> MAHHHHHHMPYQHIKVPEGGDKITVNKDFSLNVSDQPIIPYIEGDGTGFDITPVMIKVVDAAVEKAYGGKKKIHWMEIYAGEKATKVYGPDVWLPEETLQVLKEYVVSIKGPLTTPVGGGIRSLNVALRQELDLYVCLRPIQYFKGVPSPVREPEKTNMVIFRENSEDIYA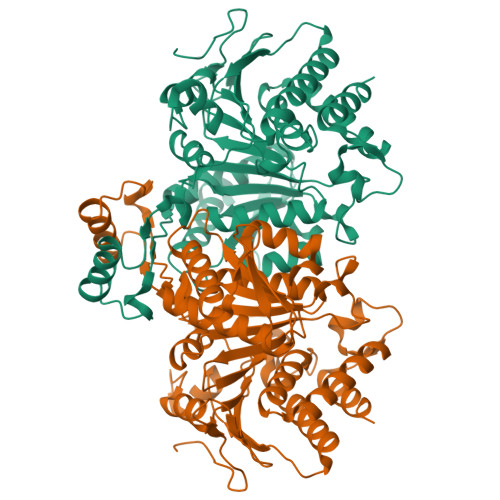GIEWAAESEQAKKVIKFLQEEMGVKKIRFPQTSGIGIKPVSKEGTERLVRKAIQYAIDNDRKSVTLVHKGNIMKFTEGAFRDAGYALAQKEFGAELIDGGPWMKFKNPKTGNEIVVKDSIADAFLQQILLRPAEYDVIATLNLNGDYISDALAAQVGGIGIAPGANLSDSVAMFEATHGTAPKYAGKDYVNPGSEILSAEMMLRHLGWTEAADVIISAMEKSIKQKRVTYDFARLMEGATQVSCSGFGQVLIENME>AKIVLVLYDAGKHAADEEK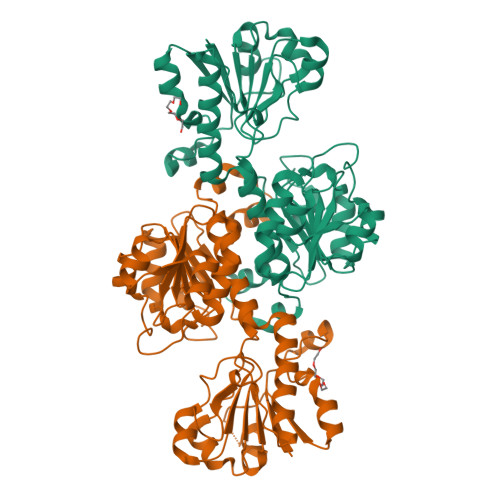LYGCTENKLGIANWLKDQGHELITTSDKEGGNSVLDQHIPDADIIITTPFHPAYITKERIDKAKKLKLVVVAGVGSDHIDLDYINQTGKKISVLEVTGSNVVSVAEHVVMTMLVLVRNFVPAHEQIINHDWEVAAIAKDAYDIEGKTIATIGAGRIGYRVLERLVPFNPKELLYYDYQALPKDAEEKVGARRVENIEELVAQADIVTVNAPLHAGTKGLINKELLSKFKKGAWLVNTARGAICVAEDVAAALESGQLRGYGGDVWFPQPAPKDHPWRDMRNKYGAGNAMTPHYSGTTLDAQTRYAQGTVNILESFFTGKFDYRPQDIILLNGEYGTKAYGKHDKK[4x]N-({4-[(2-amino-6-methyl-4-oxo-3,4-dihydrothieno[2,3-d]pyrimidin-5-yl)sulfanyl]phenyl}carbonyl)-L-glutamic 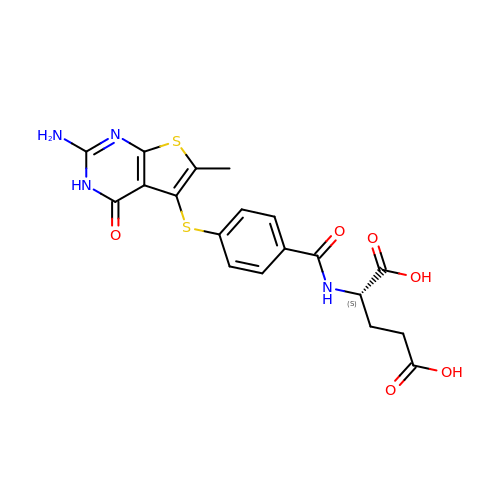acid | C19 H18 N4 O6 S2 | XZCPGLYOPFIZBL-NSHDSACASA-N Intracellular nucleotide binding, leucine-rich repeat (NLR) receptors are key components of plant innate immunity pathways. The integrated HMA domain in the sensor NLR Pik-1 directly binds the effector AVR-Pik. The Pikp NLR allele only responds to the effector variant AVR-PikD, but the Pikm allele responds to AVR-PikD, AVR-PikE, and AVR-PikA. Here, we graft an interface from Pikm onto Pikp by mutating two residues in Pikp (Asn261Lys, Lys262Glu), forming PikpNK-KE.

We found that one double mutation in two adjacent amino-acid residues contained within interface 3, Asn261Lys and Lys262Glu (henceforth PikpNK-KE), induced cell death in response to AVR-PikE and AVR-PikA. To this end, we determined the crystal structures of Pikp-HMANK-KE bound to AVR-PikD, and to AVR-PikE. Each complex was crystallized and X-ray diffraction data were collected at the Diamond Light Source (Oxford, UK) to 1.6 Å and 1.85 Å resolution, respectively. The overall architecture of these complexes is the same as that observed for all Pik-HMA/AVR-Pik effector structures. A key interaction at interface 3, one of the previously defined Pik-HMA–AVR-Pik interfaces, involves a lysine residue (Lys262 in Pikp and Pikm) that forms intimate contacts within a pocket on the effector surface. In the PikpNK-KE mutant, the position of this key lysine is shifted one residue to the N-terminus compared to that in the wild-type, so that it occupies the same position in the PikpNK-KE sequence as in the Pikm sequence. In the crystal structures of Pikp-HMANK-KE in complex with either AVR-PikD or AVR-PikE, we see that this region of the HMA adopts a Pikm-like conformation (Figure 3A, B, C and D), with no looping-out of the preceding structure. We found only limited structural perturbations at either of the other previously defined interfaces (interface 1 or 2 [De la Concepcion et al., 2018]) resulting from the binding of the AVR-PikD or AVR-PikE effectors to Pikp-HMA or Pikp-HMANK-KE. We therefore conclude that the effects of the PikpNK-KE mutant on protein function are mediated by altered interactions at interface 3.

>[4x]GPGLKQKIVIKVAMEGNNCRSKAMALVASTGGVDSVALVGDLRDKIEVVGYGIDPIKLISALRKKVGDAELLQVSQAKED;>ETGNKYIEKRAIDLSRERDPNFFDNPGIPVPECFWFMFKNNVRQDAGTCYSSWKMDMKVGPNWVHIKSDDNCNLSGDFPPGWIVLGKKRPGF[2x]> MLTNLVAEPFAKLEQDFGGSIGVYAMDTGSGATVSYRAEERFPLCSSFKGFLAAAVLARSQQQAGLLDTPIRYGKNALVPWSPISEKYLTTGMTVAELSAAAVQYSDNAAANLLLKELGGPAGLTAFMRSIGDTTFRLDRWELELNSAIPGDARDTSSPRAVTESLQKLTLGSALAAPQRQQFVDWLKGNTTGNHRIRAAVPADWAVGDKTGTCGVYGTANDYAVVWPTGRAPIVLAV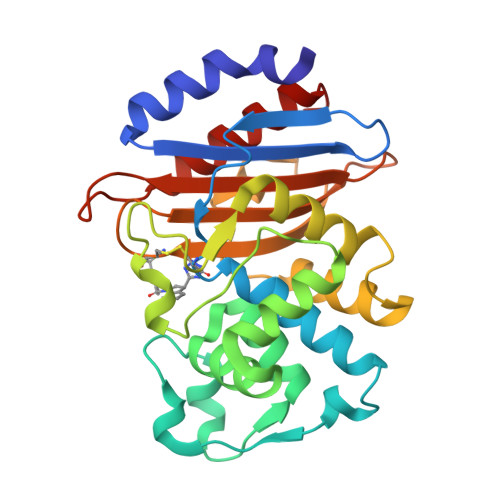YTRAPNKDDKHSEAVIAAAARLALEGLGVN> ERRRGLTDPEMAAVILKALPEAPLDGNNKMGYFVTPRWKRLTEYEALTVYAQPNADWIAGGLDWGDWTQKFHGGRPSWGNETTELRTVDWFKHRDPLRRWHAPYVKDKAEEWRYTDRFLQGYSADGQIRAMNPTWRTSSCNRYWGAFLFNEYGLFNAHSQGAREALSDVTRVSLAFWGFDKID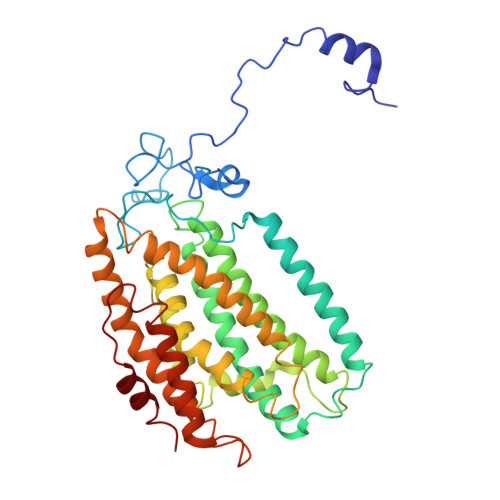IAQMIQLERGFLAKIVPGFDESTAVPKAEWTNGEVYKSARLAVEGLWQEVFDWNESAFSVHAVYDALFGQFVRREFFQRLAPRFGDNLTPFFINQAQTYFQIAKQGVQDLYYNCLGDDPEFSDYNRTVMRNWTGKWLEPTIAALRDFMGLFAKLPAGTTDKEEITASLYRVVDDWIEDYASAIDFKADRDQIVKAVLAGLK[[(2~{R},3~{S},5~{R})-5-[4-azanyl-5-[3-[2-(2-hydroxyethyloxy)ethanoylamino]prop-1-ynyl]pyrrolo[2,3-d]pyrimidin-7-yl]-3-oxidanyl-oxolan-2-yl]methoxy-oxidanyl-phosphoryl] phosphono hydrogen phosphate | C18 H26 N5 O15 P3 | 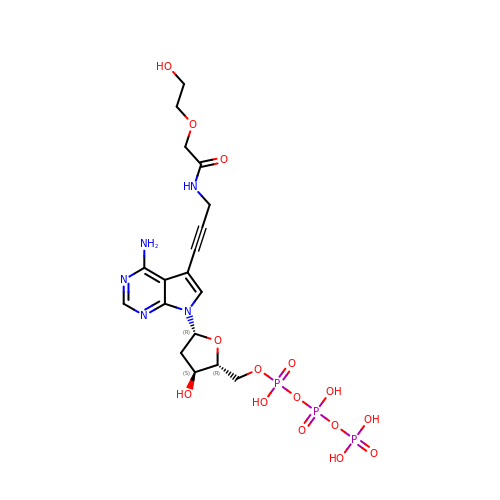FDFHIISDJKYZQH-GZBFAFLISA-N> VSLDPARTDRPYLLGRLFAVLEKAQEDAVPGANATIKDRYLASASANPGQVFHMLLK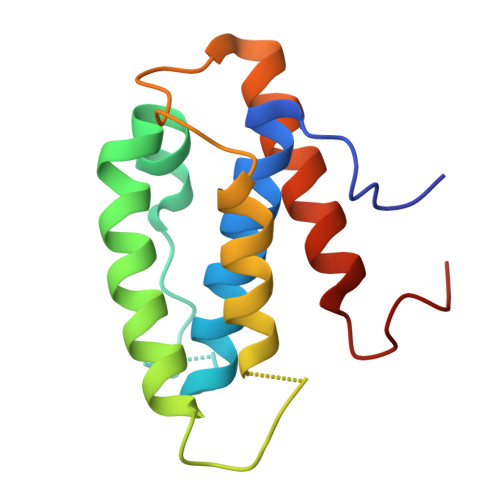NASNHTAKLRKDPERKGSAIHYEIMMQEIIDNISDFPVTMSSDEQGLFMIGYYHQRKALFTKKNKEN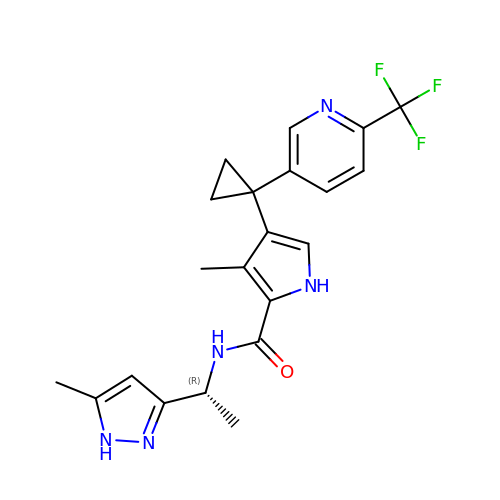3-methyl-N-[(1R)-1-(5-methyl-1H-pyrazol-3-yl)ethyl]-4-{1-[6-(trifluoromethyl)pyridin-3-yl]cyclopropyl}-1H-pyrrole-2-carboxamide | C21 H22 F3 N5 O | YRNNMQCLHYNIHR-CYBMUJFWSA-N>ELICIVQRVNESFSLHSGFGGNVYSMKTEPMTGFTNVTKGASVINQKDWIGFGDSRTDLTNDQFPASSDVPLAVAKKFRSLSGASLMLSAFGPPGKVDYLYQGCGKEKVFYEGVNWSPEAGIDCFGSNWTQTKKDFYSRIYEAARSSTCMTLVNSLDTKISSTTATAGTASSCSSSWMKSPLWYAESSVNPGAKPQVCGTEQSATFTLPTSFGIYKCNKHVVQLCYFVYENKAKFNTFGCGDYYQNYYDGNGNLIGGMDNRVAAYRGIANAGVKIECPSKILNPGTYSIKSTPRFLLVPKRSYCFDTDGGYPIQVVQSEWSASRRSDNATEEACLQTEGCIFIKKTTPYVGEADDNHGDIEMRQLLSGLGNNDTVCVSQSGYTKGETPFVKDYLSPPKYGRCQLKTDSGRIPTLPSGLIIPQAGTDS[2x];>IFGIDDLIFGLLFVGFVAGGVAGGYFWGRSNGGGGGASVSSTQAGFDKIGKDIQQLRNDTNAAIEGFNGRIAHDEQAIKNLAKEIEDARA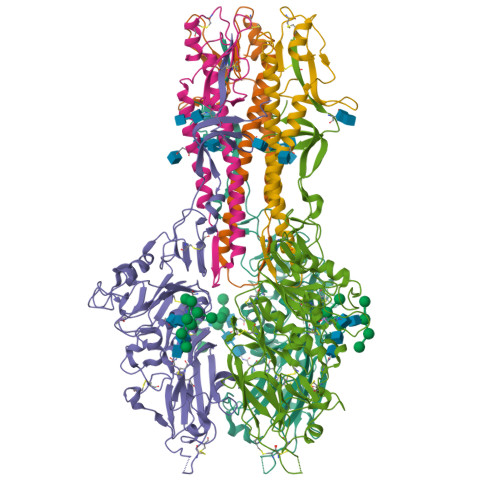EALVGELGIIRSLIVANISMNLKESLYELANQITKRGGGIAQEAGPGCWYVDSENCDASCKEYIFNFNGSATVPTL[2x]>[2x]GPEKTDEYLLARFKGDGVKYKAKLIGIDDVPDARGDKMSQDSMMKLKGMAAAGRS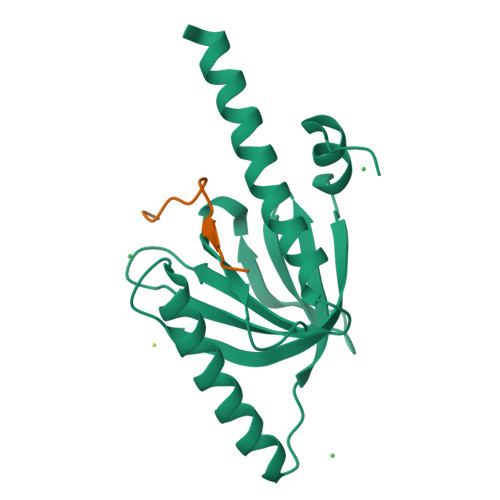QGQHKQRIWVNISLSGIKIIDEKTGVIEHEHPVNKISFIARDVTDNRAFGYVCGGEGQHQFFAIKTGQQAEPLVVDLKDLFQVIYNVKKKEEEKKKIEEASKAVEN;>XQNGFDNPNYQPQENMQA[2x]> MYDWNIAAKSQEERDKVNVDLAASGVAYKERLNIPVIAEQVAREQPENLRTYFMERLRHYRQLSL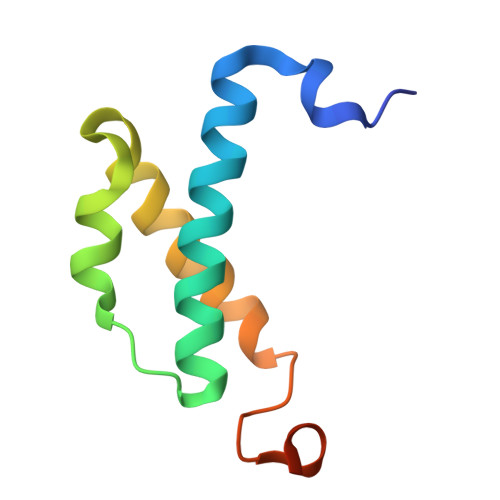QLPKGSDPAYQKDDAVKK> MNHKVHHHHHHIEGRHMKAYMFPGQGSQAKGMGRALFDAFPALTARADGVLGYSIRALCQDDPDQRLSQTQFTQPALYVVNA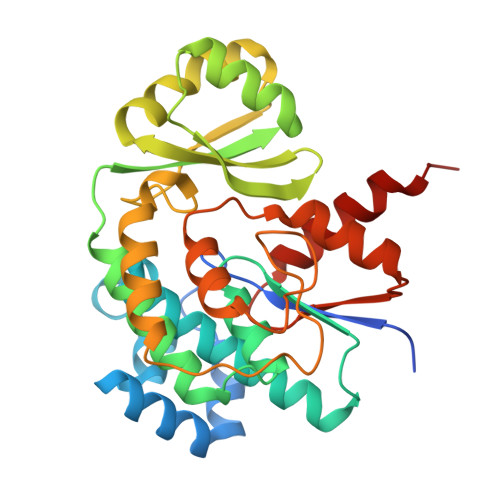LSYLKRREEEAPPDFLAGHCLGEFSALFAAGVFDFETGLALVKKRGELMGDARGGGMAAVIGLDEERVRELLDQNGATAVDIANLNSPSQVVISGAKDEIARLQVPFEAAGAKKYTVLRVSAAFHSRFMRPAMVEFGRFLEGYDFAPPKIPVISNVTARPCKADGIRAALSEQIASPVRWCESIRYLMGRGVEEFVECGHGIVLTGLYAQIRRDAQPLVV>[2x]SN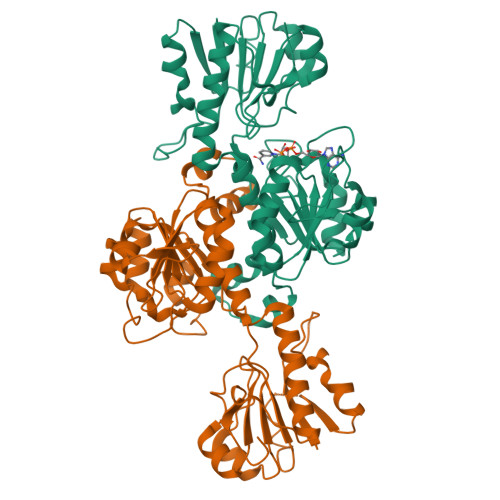GAVFFVIFLKQATCNTYFKEVKIYHLGEMDMKIVALFPEAVEGQENQLLNTKKAIGLKTFLEERGHEFIILADNGEDLDKHLPDMDVIISAPFYPAYMTRERIEKAPNLKLAITAGVGSDHVDLAAASEHNIGVVEVTGSNTVSVAEHAVMDLLILLRNYEEGHRQSVEGEWNLSQVGNHAHELQHKTIGIFGFGRIGQLVAERLAPFNVTLQHYDPINQQDHKLSKFVSFDELVSSSDAITIHAPLTPETDNLFDKDVLSRMKKHSYLVNTARGKIVNRDALVEALASEHLQGYAGDVWYPQPAPADHPWRTMPRNAMTVHYSGMTLEAQKRIEDGVKDILERFFNHEPFQDKDIIVASGRIASKSYTAK>MGSDKIHHHHHHMYVTSQIHAKGSDLAKLMQIAALKGNEEVLDVATGGGHVANAFAPFVKKVVAFDLTEDILKVARAFIEGNGHQQVEYVQGDAEQMPFTDERFHIVTCRIAAHHFPNPASFVSEAYRVLKKGGQLLLVDNSAPENDAFDVFYNYVEKERDYSHHRAWKKSDWLKMLEEAGFELEELHCFHKTFIFEDWCDRMNVTTEKKQELSDFIKSKPTEYYQKFKIVVEDGRVYSFRGESILMKARKPTVKN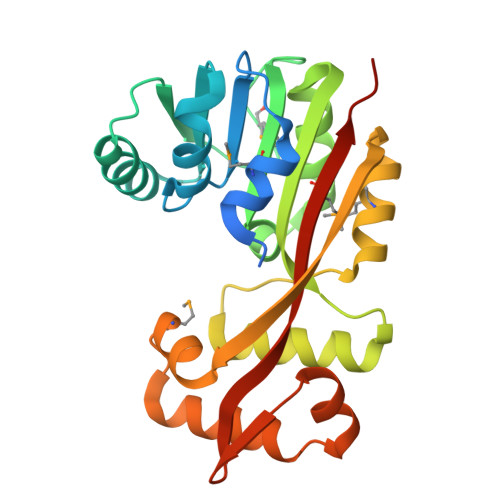KGSS[4x]> MNIVLMGLPGAGKGTQADRIVEKYGIPHISTGDMFRAAIQEGTELGVKAKSFMDQGALVPDEVTIGIVRERLSKSDCDNGFLLDGFPRTVPQAEALDQLLADMGRKIEHVLNIQVEKEELIARLTGRRICKVCGTSYHLLFNPPQVEGKCDKDGGELYQRADDNPDTVTNRLEVNMNQTAPLLAFYDSKEVLVNINGQKDIKDVFKDLDVILQGNGQ

Adenylate kinase (AK) is a phosphotransferase enzyme catalyzing interconversion between ATP/AMP and two ADPs and is inhibited by P1,P5-di(adenosine 5′)-pentaphosphate (Ap5A), which mimics two adenylate substrates. Structural studies have revealed three characteristic AK domains, namely, the CORE, AMPbind, and LID domains. In the present study, a structural comparison of AKp and AKm revealed suboptimal hydrophobic packing in the CORE domain of the psychrophilic homologue, where a polar side chain makes contact with hydrophobic neighboring residues. We also determined the crystal structures of two AK mutants, which showed the largest thermal stability transition compared to wild-type (WT) AKs.

The psychrophilic AKp contains a more polar Thr26 instead of the Ile residue. In the structure-based sequence alignment, we found that other AKs also contain hydrophobic residues in the positions equivalent to Thr26 and the five neighboring residues in AKp. These observations strongly suggest that Thr26 in AKp disrupts hydrophobic packing in the CORE domain and likely decreases its thermal stability compared to other AKs including AKm. Consistent with this, the Thr-to-Ile substitution at residue 26 significantly increased the thermal stability of psychrophilic AKp, as indicated by a Tm value of 8.1 °C higher than the WT protein. The AKp T26I mutant showed increased catalytic activities at high temperatures (55 and 65 °C) compared to WT enzyme, and the temperature of maximum activity shifted from 45 °C to 55 °C by the mutation. Interestingly, the Thr-to-Ile mutation did not significantly affect the catalytic activity of AKp at relatively low temperatures (5 °C to 45 °C). In the structure of the T26I mutant of AKp, the side chain of Ile26 adopts a conformation almost identical to that of Ile26 in WT AKm and interacts closely with the neighboring hydrophobic CORE residues, as in the WT mesophilic homologue. The AKp I26T mutant has increased the apolar buried surface area compared to WT, and almost half of the increase resulted from the six-residue cluster including Ile26 and the five neighboring residues. The T26I mutant of AKp shows an average B-factor (50.0 Å2) similar to that of WT AKp (51.4 Å2) for all protein atoms (residues 1–213), whereas the average value for atoms of Ile26 (53.0 Å2) in the mutant is considerably smaller than that of Thr26 (60.7 Å2) in the WT structure, even though the side chain of Ile is longer than that of Thr. These observations suggest that the flexibility of residue 26 is decreased by Thr-to-Ile substitution in AKp, and the relative rigidity of the mutated Ile26 likely results from enhanced hydrophobic interactions with neighboring residues in the CORE domain. Our structural and mutational analyses indicated that the significant thermal stabilization observed in the T26I mutant of AKp resulted from optimization of the hydrophobic CORE packing.>[4x]MSNTE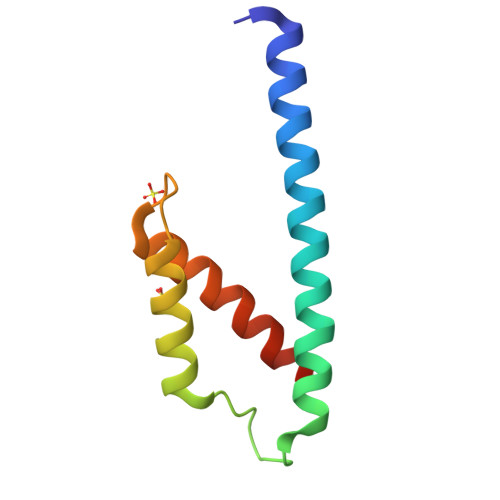LELLRQKADELNLQILKLINERGNVVKEIGKAKEAQGVNRFDPVRERTMLNNIIENNDGPFENSTIQHIFKEIFKAGLELQEEDH>MAHHTKETMELIKELVSIPSPSGNTAKIINFIENYVSEWNVETKRNNKGALILTVKGKNDAQHRLLTAHVDTLGAMVKEIKPDGRLSLSMIGGFRWNSVEGEYCEIETSSGKTYTGTILMHQTSVHVYKDAGEAKRDEKNIEVRIDERVFSADEVRELGIEVGDFVSFDPRVQITESGYIKSRHLDDKVSVAILLKLIKRLQDENVTLPYTTHFLISNNEEIGYGGNSNIPEETVEYLAVDMGALGDGQASDEYTVSICAKDSSGPYHYALRKHLVELAKTNHIEYKVDIYPYYGSDASAAIRAGFDVKHALIGAGIDSSHAFERTHES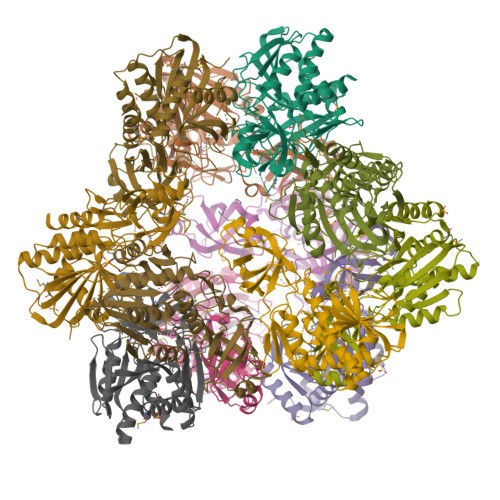SIAHTEALVYAYVMSNLIEE[16x]>AGSGHMMELHILEHRVRVLSVARPGLWLYTHPLIKLLFLPRRSRCKFFSLTETPEDYTLMVDEEGFKELPPSEFLQVAEATWLVLNVSSHSGAAVQAAGVTKIARSVIAPLAEHHVSVLMLSTYQTDFILVREQDLSVVIHTLAQEFDIYREVGGEPVPVTRDDSSNGFPRTQHGPSPTVHPIQSPQNRFCVLTLDPETLPAIATTLIDVLFYSHSTPK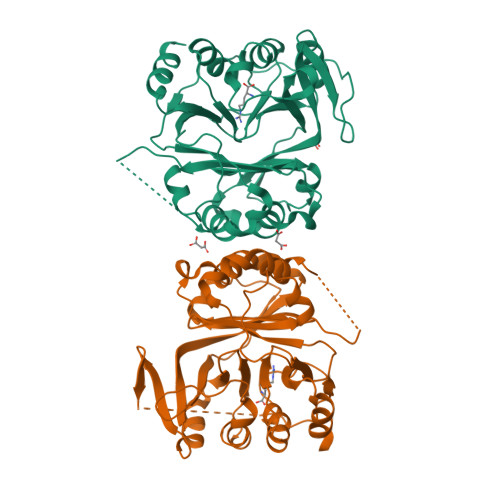EAASSSPEPSSITFFAFSLIEGYISIVMDAETQKKFPSDLLLTSSSGELWRMVRIGGQPLGFDECGIVAQIAGPLAAADISAYYISTFNFDHALVPEDGIGSVIEVLQRRQEGLAS[4x]>[4x]EEKKKKRSGFRDRKVMEYENRIRAYSTPDKIFRYFATLKVISEPGEAEVFMTPEDFVRSITPNEKQPEHLGLDQYIIKRFDGKKISQEREKFADEGSIFYTLGECGLISFSDYIFLTTVLSTPQRNFEIAFKMFDLNGDGEVDMEEFEQVQSIIRSQTSMGMRHRDRPTTGNTLKSGLCSALTTYFFGADLKGKLTIKNFLEFQRKLQHDVLKLEFERHDPVDGRITERQFGGMLLAYSGVQSKKLTAMQRQLKKHFKEGKGLTFQEVENFFTFLKNINDVDTALSFYHMAGASLDKVTMQQVARTVAKVELSDHVCDVVFALFDCDGNGELSNKEFVSIMKQRLMRG;>HHHHHHMSLRKQRFMQFSSLEHEGEYYMTPRDFLFSVMFEQMERKTSVKKLTKKDIEDTLSGIQTAGCGSTFFRDLGDKGLISYTEYLFLLTILTKPHSGFHVAFKMLDTD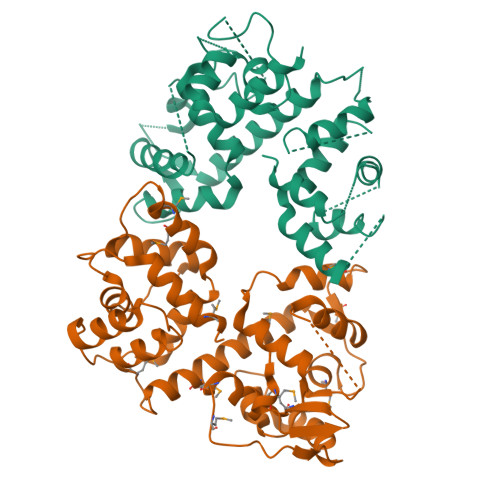GNEMIEKREFFKLQKIISKQDDLMTVKTNETGYQEAIVKEPEINTTLQMRFFGKRGQRKLHYKEFRRFMENLQTEIQEMEFLQFSKGLSFMRKEDFAEWLLFFTNTENKDIYWKNVREKLSAGESISLDEFKSFCHFTTHLEDFAIAMQMFSLAHRPVRLAEFKRAVKVATGQELSNNILDTVFKIFDLDGDECLSHEEFLGVLKNRMHRGLWV[4x]>TWRDFGRKLRLLSGYLWPRGSPALQLVVLICLGLMGLERALNVLVPIFYRNIVNLLTEKAPWNSLAWTVTSYVFLKFLQGGGTGSTGFVSNLRTFLWIRVQQFTSRRVELLIFSHLHELSLRWHLGRRTGEVLRIADRGTSSVTGLLSYLVFNVIPTLADIIIGIIYFSMFFNAWFGLIVFLCMSLYLTLTIVVTEWRTKFRRAMNTQENATRARAVDSLLNFETVKYYNAESYEVERYREAIIKYQGLEWKSSASLVLLNQTQNLVIGLGLLAGSLLCAYFVTEQKLQVGDYVLFGTYIIQLYMPLNAFGTYYRMIQTNFIDMENMFDLLKEETEVKDLPGAGPLRFQKGRIEFENVHFSYADGRETLQDVSFTVMPGQTLALVGPSGAGKSTILRLLFRFYDISSGCIRIDGQDISQVTQASLRSHIGVVPQDTVLFNDTIADNIRYGRVTAGNDEVEAAAQAAGIHDAIMAFPEGYRTQVGERGLKLSGGEKQRVAIARTILKAPGIILLDEATSALDTSNERAIQASLAKVCANRTTIVVAHRLSTVVNADQILVIKDGCIVERGRHEALLSRGGVYADMWQLQQG[2x]

Human ATP-binding cassette transporter subfamily B6 (ABCB6) is a mitochondrial porphyrin transporter that uses energy from ATP hydrolysis to translocate the heme precursors protoporphyrin IX and coproporphyrinogen III from the cytoplasm into mitochondria for heme biosynthesis. ABCB6 is a Type IV half-transporter of 842 amino acids with only one transmembrane domain (TMD) and one cytosolic nucleotide-binding domain (NBD) with an extra N-terminal TMD (TMD0). It functions as a homodimer with the substrate transport pathway and the active site of ATP hydrolysis built from residues from both chains. Within the transport pathway, a conserved aromatic residue W546 located in each monomer plays a pivotal role in stabilizing the occluded conformation via π-stacking interactions.

Notably, in the post-occluded state, we observed strong electron density within a hydrophobic groove formed by the elbow helix, TM 9, and TM 11 of each monomer. The density shape corresponds to a phospholipid molecule with two fatty acyl chains. Therefore, we constructed an atomic model of the POPE (or 16:0-18:1 PE) molecule in the head-down orientation as a representative phospholipid model. Our analysis revealed that POPE interacts with highly conserved residues across species. Furthermore, given the presence of a similar lipid density in the pre-occluded state, it is evident that a phospholipid bound to the TMD groove acts as a ‘wedge’ to stabilize the occlusion state of the transporter. Collectively, our findings suggest that direct protein-lipid interactions contribute to the increase in the relative stability of the inward-facing or occluded states. Structural analysis suggests that the lipid inserted within the TMD groove may compensate for the W546A mutation by acting as a molecular wedge to resist conformational transitions to the outward-facing form. In the lipid environment, however, the transporter predominantly adopted the post-occluded state irrespective of the presence of the W546A mutation. Formation of the post-occluded state after substrate release reorients the TMDs closer together at the two-fold dimer axis such that the central cavity is no longer present (lower left).> KKPPTVVQSRTDVFNEQFANEALHPMTKVIFNGLDVNTEVQPLSDDFKQISDPKGYLTYSVKYEDQFTKKDKLRASEADDRIVGPTVNLFKYGAAVVNIDLNRDFFDTATGIDLTKGIPLVQDLLVPIGVTAGAEQSAEYVSGLLMVLFKVMTDNRLVIVGETTTPMSNTLSTVVNNVLRTTYHNNVGVNPALLRDFTQVNWLNRDITNMLQQAGTKYGLGLTETRLDYVRLVKTIVGHALNIDHFAASVLNINLRALMEANVTADD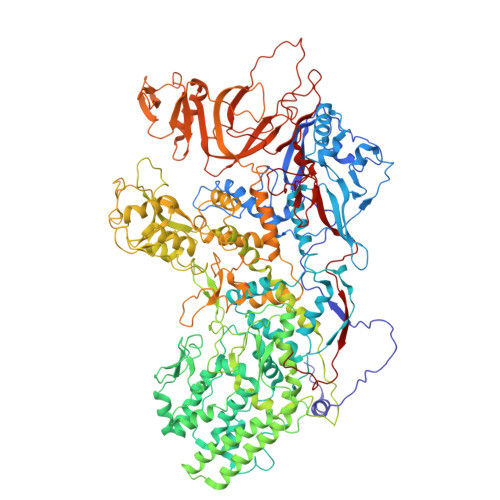RIKALQAHSMISTQFHGPNQGALRPELAFDHDHIIRCLMLAAANYPRLEGIIVQINTGYVASANVIRPVSEKRYFPENLEQNQSAARLVSAVKARASEADISSIHLAIAREVSPMFNVHELKKIAESFEDPSSIVVVLEFILFALFFPTEFNRIKGDIQNVLLLFFSRWYPVEYGIFIQRGATYTINAAGEFEFSGRNEKWDQSLYLSEHFPALFSDVPLAGANTIIAIMRLFTPQGFLRTDDLAIAANFPRASRNPQTYIPYTNQRGTVTNEFASRFRTIVATLANVVNERAVQDDMQKATRSCTKQWLRHLETQFDNIAVAHTDHLSVVYATMSNFMLNFTNNFSGNHATFKPDQYVITSPEGSYKPIIERQGETVDGLTIIDTSIVWPILCQCTYPLVRQSGKGVDAVSIMEEIVYPDPSTTLSQSLSVAQVLSKLTLPDAFINMILSGGDSVVMRTYQTEADDDLDEGIRMTTYDQYLSHIRERLHITNVPDPIYITGASTPDQIAASVQATHVAVVLYQSGVINGSASTYLRENEVLVVMPDYYDVVSRFANANLQMNNNRYHESVLEIADIFDQADFIQTSDAVRQLRALMPTLSTSQIRHAIERIAQITDVDSTDYGKLTLRFLGTLTRSLKMQNAQIRRIRPDGTVLRYDDQIDIEAFRWSRYFLDELRLRRLSVGLRLITNPRIARRFDGVRIMYLTDDDPDPDFVPDVPEGYVAVQYAHRLFSSSLANKRNRVTYTHPPTGMAYPSPTGRPHVHMTINERAGMSKLVADNIIASVIKSNWVVDIHDIEYTAEVMTPSEGYTQHVDAESIMTAPKGKLFHLQFMDGLLRPEPSAFDPPASGEDMRLIYPLQPISVARSMRAIVNHNEVDRPRGAVAPSSYEMDTGTLSRNGDLLYSPVANGQVGIPKLEVDHISFSNVVSMMTANIRTGDDMAVERVNPDDVRAINIRNA> VAFGSEDIENTLAKMDDGQLDGLAFGAIQLDGDGNILQYNAAEGDITGRDPKQVIGKNFFKDVAPCTDSPEFYGKFKEGV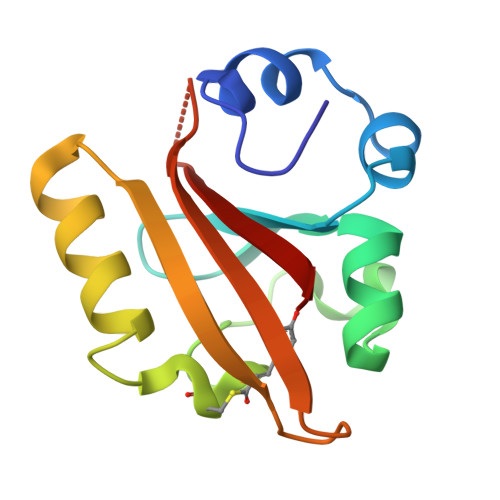ASGNLNTMFEYTFDYQMTPTKVKVHMKKALSGDSYWVFVKRV> MAYADRYDAAFGIYISRFLRNNVHTNIRGKVVGVNYSG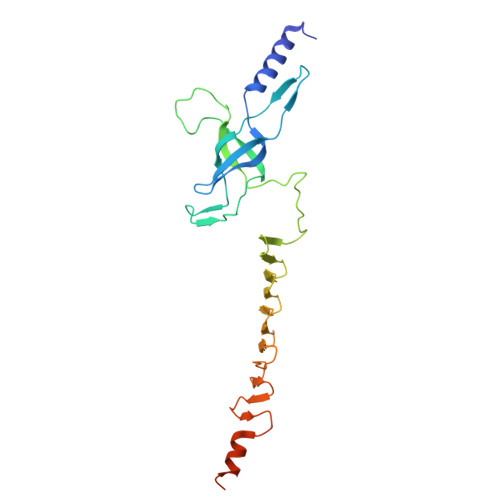PSVDVQPMAYTEFPSGTTDRYPVIYDVPVLLPSGAGGKARLTMPIKPGDVVGLSFSERNEGDNNDQNTHQLFAGWAVTQIFTDGNSKAIHPDNVVLENDKAIITLKPDGDTSLQNPKVTVEALADGNVKISNGTGEFTMSPSGEIKGGNRGGSFTLQPSGQLMCNGARITTSGRIITANGVDMDDFYQKYMSHTHGGVSRGGDNTNPPN(3R,3aR,6aS)-N-[(4R,7S,8S,10R,13S)-8-hydroxy-10,17-dimethyl-7-(2-methylpropyl)-5,11,14-trioxo-13-(propan-2-yl)-2-thia-6,12,15-triazaoctadecan-4-yl]hexahydrofuro[3,2-d][1,2]oxazole-3-carboxamide 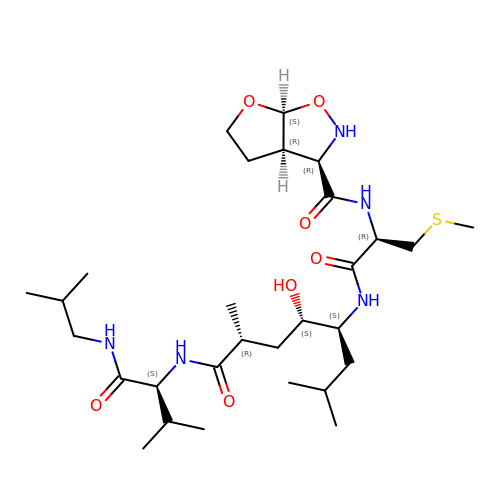| C29 H53 N5 O7 S | FHZUZMVZKPPWHG-VRUQXOILSA-N> INTITFDAGNATINKYATFMESLRNEAKDPSLKCYGIPMLPNTNSTIKYLLVKLQGASLKTITLILRRNNLYVMGYSDPYDNKCRYHIFNDIKGTEYSDVENTLCPSTNPRVAKPINYNGLYPTLENKAGVTSRNQVQLGIQILSSDIGKISGQGSFTEKTEAKFLLVAIQMVPEAARFKYIENQVKTNFNRDFFPNDKVLELEENWGKISTAIHDAKNGALPKPLELKNADGTKWIVLRVDEIKPDVGLLKYVNGTCQ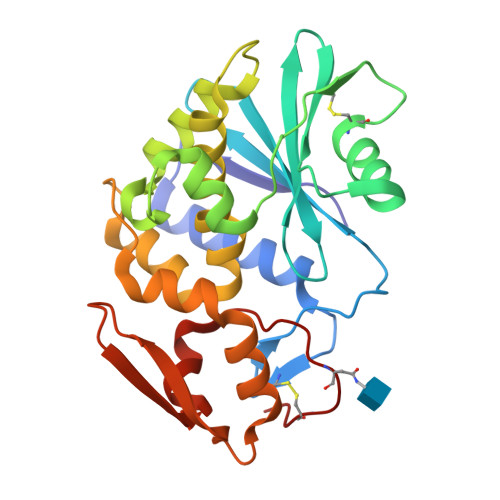TT> SLGSLTIAEPAMIAECKTRTEVFEISRRLI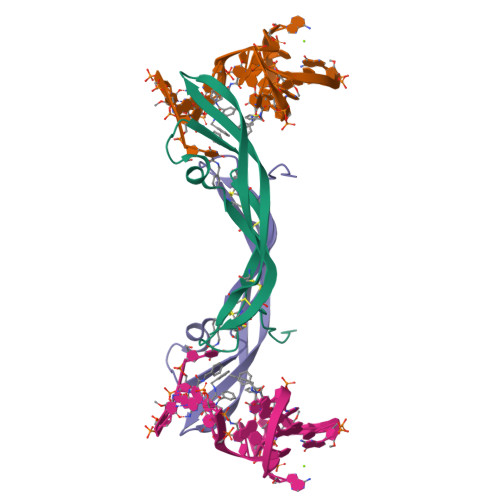DRTNANFLVWPPCVEVQRCSGCCNNRNVQCRPTQVQLRPVQVRKIEIVRKKPIFKKATVTLEDHLACKCETVAAARPVT>[2x]MPGRRKACFVTALTSRTELDIDPDKLRESVVELLERHPLVFEGTRQLALQHRPEATDPWYEGCQRQSLISSDSDFTEVHGE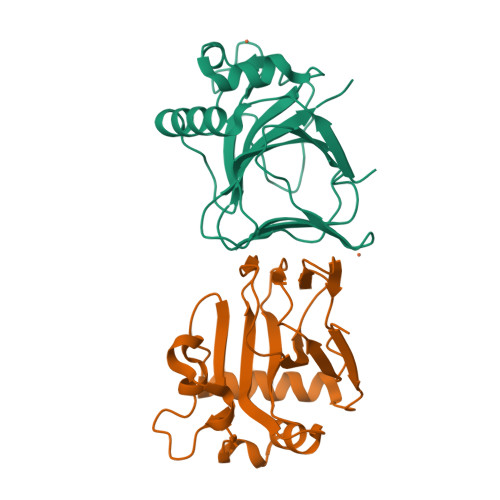LRDTYLGEVFDRLPFKPIRTRIMALDPKYCYSVHRDLTPRYHLAVTTSEHARFVFIEHDKVLHIPADGDLYYVDTRQLHSAFNGGDDMRIHIVFGTDGESK> TVILEYAHRL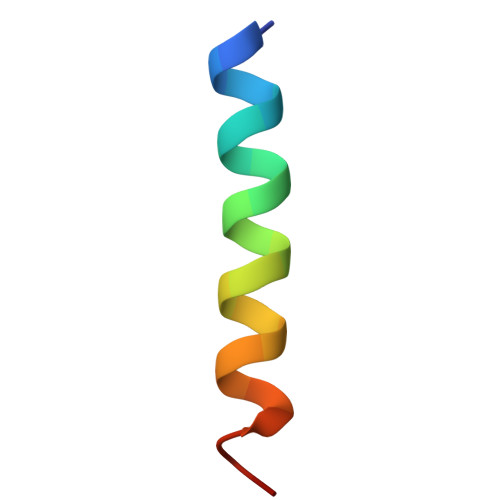SQDILCDALQQWAC> GSMNTHPPQLMEATSAKIVMLGESGAGKSSIALRFTRNEFLANQETTIGAAFLSKTVMIDGRALKYEIWDTAGLERFRSLAPIYYRGASGALVVYDITNSESLKKAQTWIKELRANADPSL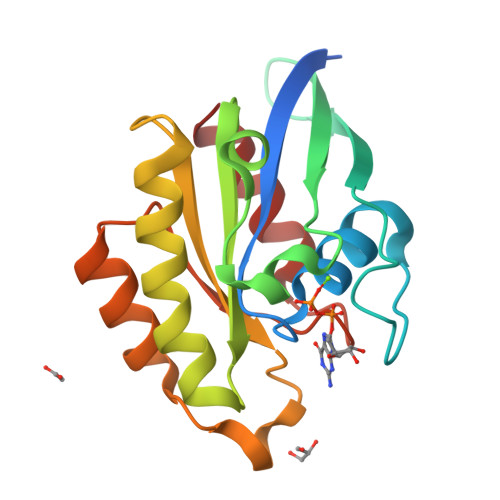IIVLVGNKKDLGSLRQVSFEDGQRLAAEEQLAAFYEASAKDNNNVEQVFLDLAAKL>MTIYVVTPTYARLVQKAELVRLSQTLSLVPRLHWLLVEDAEGPTPLVSGLLAASGLLFTHLVVLTPKAQRLREGEPGWVHPRGVEQRNKALDWLRGRGGAVGGEKDPPPPGTQGVVYFADDDNTYSRELFEEMRWTRGVSVWPVGLVGGLR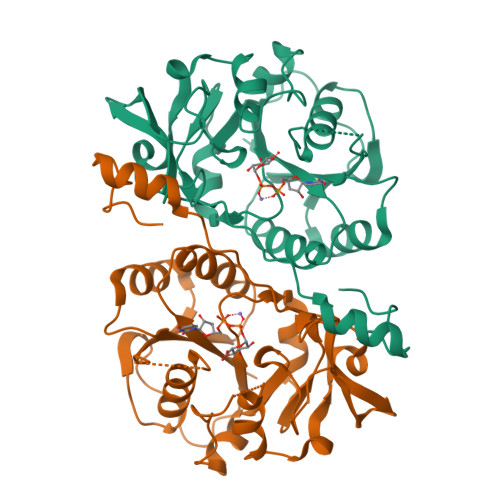FEGPQVQDGRVVGFHTAWEPSRPFPVDMAGFAVALPLLLDKPNAQFDSTAPRGHLESSLLSHLVDPKDLEPRAANCTRVLVWHTRTEKPKMKQEEQLQRQGRGSDPAIEV[2x]> MPREIITLQLGQCGNQIGFEFWKQLCAEHGISPEAIVEEFATEGTDRKDVFFYQADDEHYIPRAVLLDLEPRVIHSILNSPYAKLYNPENIYLSEHGGGAGNNWASGFSQGEKIHEDIFDIIDREADGSDSLEGFVLCHSIAGGTGSGLGSYLLERLNDRYPKKLVQTYSVFPNQDEMSDVVVQPYNSLLTLKRLTQNADCLVVLDNTALNRIATDRLHIQNPSFSQINQLVSTIMSASTTT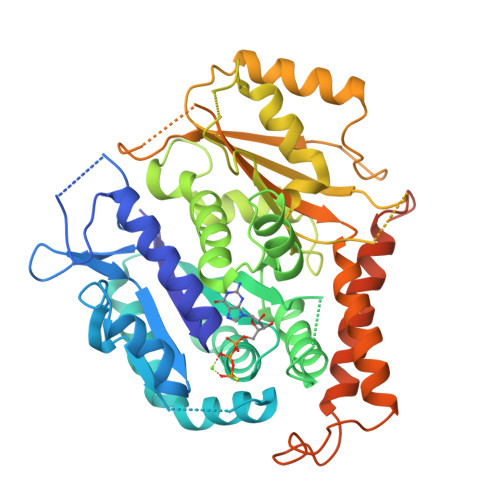LRYPGYMNNDLIGLIASLIPTPRLHFLMTGYTPLTTDQSVASVRKTTVLDVMRRLLQPKNVMVSTGRDRQTNHCYIAILNIIQGEVDPTQVHKSLQRIRERKLANFIPWGPASIQVALSRKSPYLPSAHRVSGLMMANHTSISSLFERTCRQYDKLRKREAFLEQFRKEDMFKDNFDEMDTSREIVQQLIDEYHAATRPDYISWGTQVDVDGGEQKLISEEDLLLEHHHHHH One of the major and widespread PTMs is acylation of the ε-amino group of lysine residues. Canonical acyllysine readers, bromodomain and double PHD finger (DPF), display comparable binding capabilities toward various short acyl chain modifications, and while the YEATS domain exhibits preference for crotonyllysine, it still associates albeit more weakly with other acyllysine marks. In this study, we elucidate the significance of π stacking components in targeting of acetyllysines by the YEATS domains and report a previously uncharacterized DNA-binding activity of the human AF9-YEATS domain. Collectively, our results have illuminated the mechanistic basis underlying distinct recognition of acyllysine PTMs by the YEATS domains of yeast Taf14 and human AF9, allowing us to develop a Taf14-YEATS module that selects for the crotonyl modification and discriminates against saturated acyl modifications.

Alignment of the YEATS domain sequences derived from the family of human and yeast proteins shows conservation of the WG motif (W81 and G82 in Taf14) in all YEATS members but AF9 and ENL, which instead contain a YA motif. To compare the binding modes of the YEATS domains harboring the WG and YA motifs, we determined the structure of AF9-YEATS in complex with H3K9bu peptide. Structural overlay of the AF9-YEATS:H3K9bu and previously reported AF9-YEATS:H3K9cr17 complexes showed that both saturated and unsaturated four-carbon acyl chains of K9 are bound by the three aromatic residues Y78, F59, and F28 in a very similar way. Short (<4 Å) distances observed between Cγ, Cδ, Cε, and Cη atoms of Y78, the amide group of acyllysine, and the Cε and Cζ atoms of F59 indicated that Y78 and F59 of AF9 are involved in the aromatic-amide-aromatic π-π-π stacking in either complex (yellow dashed lines). However, neither Y78 nor F28 appear to form π-π-π stacking with the alkene group of crotonyllysine as only a single carbon atom in Y78 (Cε) or F28 (Cε) was close enough to the C = C carbon atoms to fully engage the double bond (red dashed lines). This inability to form the additional energetically favorable contact is likely the reason behind the indifference of the YEATS domain of AF9 toward crotonyl-, butyryl-, and acetyl-H3K9acyl modifications.

>GSHMASSCAVQVKLELGHRAQVRKKPTVEGFTHDWMVFVRGPEHSNIQHFVEKVVFHLHESFPRPKRVCKDPPYKVEESGYAGFILPIEVYFKNKEEPRKVRFDYDLFLHLEGHPPVNHLRCEKLTFNNPTEDFRRKLLKA[2x];>[2x]ARTKQTARXSTGGKAPRKQ> MDEFEMIKRNTSEIISEEELREVLKKDEKSALIGFEPSGKIHLGHYLQIKKMIDLQNAGFDIIILLADLHAYLNQKGELDEIRKIGDYNKKVFEAMGLKAKYVYGSSFQLDKDYTLNVYRLALKTTLKRARRSMELIAREDENPKVAEVIY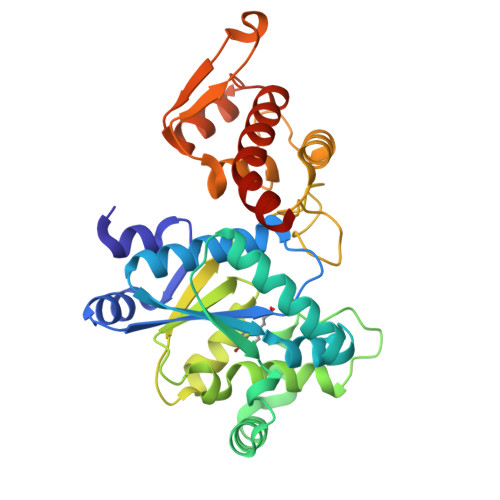PIMQVNPLHYEGVDVAVGGMEQRKIHMLARELLPKKVVCIHNPVLTGLDGEGKMSSSKGNFIAVDDSPEEIRAKIKKAYCPAGVVEGNPIMEIAKYFLEYPLTIKRPEKFGGDLTVNSYEELESLFKNKELHPMDLKNAVAEELIKILEPIRKRLLEHHHHHH>[6x]SNAMTNIIKIRASVFIPMSWTEA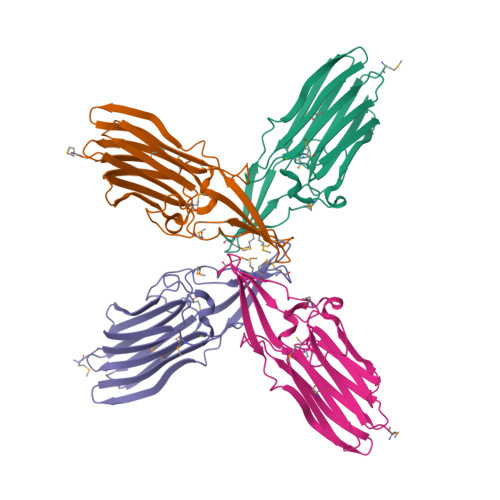KMDMETGQVIQFEGDSREFTPHAVNTMRSRVEQEVVVDFYKQEVFSYANTGITTEKVISPDGSVNKRTGKASTENIVCTDIVWNSGGVQFKMSASASNPLNVYAPPVDYVLNVCVKKDGSIDVQGEHDGFPCFEFYKQVDFGPFEKIYTHDFRETGDTAAALGGNMDYSFTKRL> GGLEKDFLPLYFGWFLTKKSSETLRKAGQVFLEELGNHKAFKKELRHFISGDEPKEKLELVSYFGKRPPGVLHCTTKFCDYGKAAGAEEYAQQEVVKRSYGKAFKLSISALFVTPKTAGAQVVLTDQELQLWPSDLDKPSASEGLPPGSQAHVTLGCAADVQPVQTGLDLLDILQQVKGGSQGEAVGELPRGKLYSLGKGRWMLSLTKKMEVKAIFTGYYG

2′,3′-cyclic nucleotide 3′-phosphodiesterase (CNPase) comprises 4% of total myelin protein in the central nervous system (CNS), being the most abundant CNS non-compact myelin protein4. CNPase consists of an N-terminal polynucleotide kinase-like domain10, a catalytic phosphodiesterase domain11, and a membrane-anchored C-terminal tail, which contains a cysteine residue that undergoes isoprenylation. The catalytic domain enables the rapid hydrolysis of nucleoside 2′,3′-cyclic phosphates to nucleoside 2′-phosphates. The CNPase catalytic site, lying in a groove between two lobes, has pseudo two-fold symmetry and contains two apposing His-X-Thr-X (X denotes a hydrophobic residue) motifs, characteristic for 2H phosphoesterases 113537.

In the vicinity of the bound nucleotide and the catalytic core, the side chain of Arg307 can swing towards and away from the active site and, therefore, could play a role in the catalytic cycle. The complex with adenosine 2′-monophosphate (2′-AMP) reveals that the R307Q mutant binds the product in a mixed conformation, whereby only the phosphate position changes, and the β5-α7 loop also presents a linked double open/closed conformation. Also, similarly to V321A, R307Q presents an elevated KM, while kcat remains at the wild-type enzyme level. While Arg307 can be assumed to mainly affect ligand binding affinity, its mode of action is not entirely clear, as Arg307 makes no direct interactions with active site ligands in crystal structures. Arg307 may be important for active-site electrostatics, likely playing a role in attracting substrates to bind. In the substrate complex34, Arg307 is positioned towards the active site, like in the wild-type CNPcat apo structure, whereas in R307Q, Gln307 is turned away – quite similarly to Arg307 in P296G complexed with 2′-AMP (see next paragraph), and notably, in the sulphate complex determined earlier, where wild-type CNPcat coordinates a sulphate ion at the nearby anion binding pocket. Gln307 similarly coordinates a chloride ion in the anion binding pocket, together with Trp289 and the backbone amide of Gly305. In all structures, the 2.8-Å hydrogen bond between His230 Nδ1 and the carbonyl O of residue 307 is retained, which results in a ~1 Å retraction of the main chain at position 307 in the sulphate complex38 and R307Q. During catalysis, the β5-α7 loop opens to expose the N terminus of helix α7 and to provide space for the product, which still remains locked in a very similar orientation as the original substrate. This loop opening might be modulated by the conformation of Arg307, since our R307Q structure demonstrates that in the absence of Arg307, the loop apparently has a much higher degree of freedom and adopts a mixed open/closed conformation.>[2x]GMAEEQNPSATFDTILTLDFGSQYTHLITRRLREIGVYSEMLPCTQKLADLPFKPKGIILSGGPYSVYEDGAPHADPAVFELGVPVLGICYGLQEIAYRLGKDNVVAGTAREYGHADLNAQRLDNQGHVDKLFAGLEEHVKVWMSHGDKLVKLPEGFHTIATTANSEYAGIAHETKPVYGIQFHPEVTHTPDGAKLLRNFAVDICGANP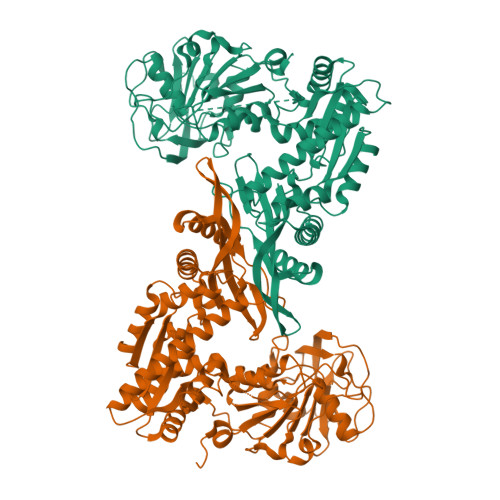NWTMSKFVDQEILRIRKLVGETDHVLGAVSGGVDSTVAAKLMKEAIGDRFHAVLVNNGCMRLNECETVAETLNKHLGINLTVVDASKRFLDGLKGVTDPEKKRMFIGATFIDVFEEEAEKIEALAENSGAKVKWFLQGTLYPDVIESISFKGPSATIKTHHNVGALPKRMIEGQGMKLIEPLRELFKDEVRQLGRELGIAHELVMRHPFPGPGIAIRVLGEVTPERVDIARKADHIFISMIREAGLYDKISQAYAALDPSKAVGVMGDKRVYAEIIILRAVETTDFMTARAFPFDNEFLSKCATRIINEVHGVSRVLYDISSKPPATIEME> AKPIDVSRLDLRI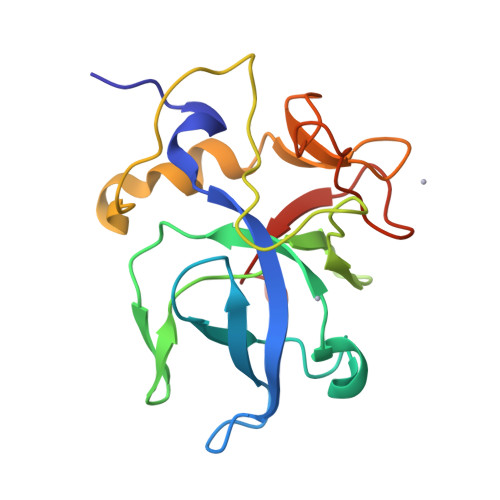GCIITARKHPDADSLYVEEVDVGEIAPRTVVSGLVNHVPLEQMQNRMVILLCNLKPAKMRGVLSQAMVMCASSPEKIEILAPPNGSVPGDRITFDAFPGEPDKELNPKKKIWEQIQPDLHTNDECVATYKGVPFEVKGKGVCRAQTMSNSGIKLEHHHHHH> GSPPARKEKTKVKESVSRVEKAKQKSAQQELKQRQRAEIYALNRVMTEL;> MDEATWERMWKHVAKIHPDGEKVA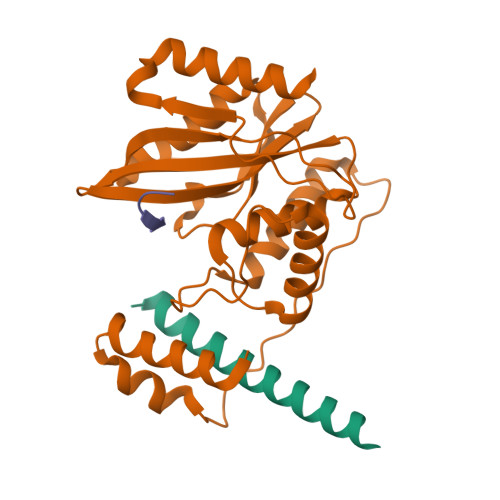QRIRGATDLPKIPIPSVPTFQPSTPVPERLEAVQRYIRELQYNHTGTQFFEIKKSRPLTGLMDLAKEMTKEALPIKSLEAVILGIYLTNSMPTLERFPISFKTYFSGNYFRHIVLGVNFAGRYGALGMSRREDLMYKPPAFRTLSELVLDFEAAYGRCWHVLKKVKLGQSVSHDPHSVEQIEWKHSVLDVERLGRDDFRKELERHARDMRLKIG;> GEEEGEEY> 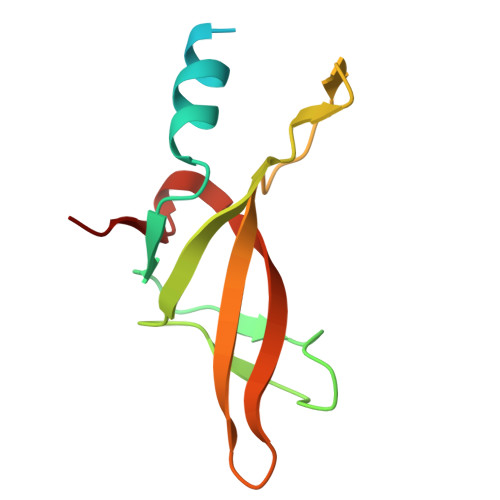DIAVKSAASVDADADLSSSTSLETEEDEKAKEKIGARVRVTVPLKVYHVVRVPEVELMGMEGFIKDYVVLWKGKKISANLPFKVQFVKEIEGRGPVKFFTHLKEDEFELIDP>VESLMQALPGIGWTAALLLMMFYIFAVMGTELFGEAFPQWFGSLGASIYSLFQIMTLESWSMGIARPVMEVYPLAWIFFVPFILISSFMVLNLFIAIIVSATQE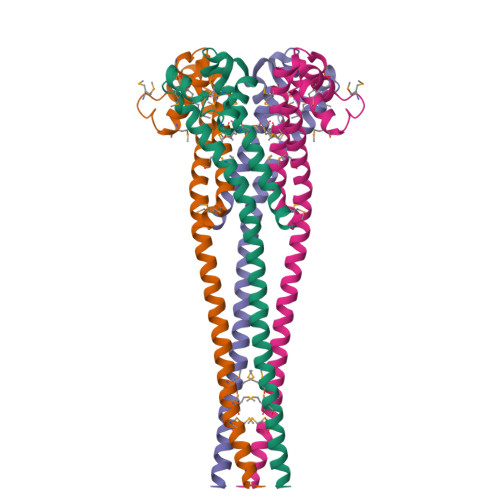VHESEQRAEREANNLIAHDERQEMLDLMRAMHAKIVALEQQGA[2x]> KPEPTDEEWELIKTVTEAHVATNAQGSHWKQKRKFLPEDIGQAPIVNAPEGGKVDLEAFSHFTKIITPAITRVVDFAKKLPMFCELPCEDQIILLKGCCMEIMSLRAAVRYDPESET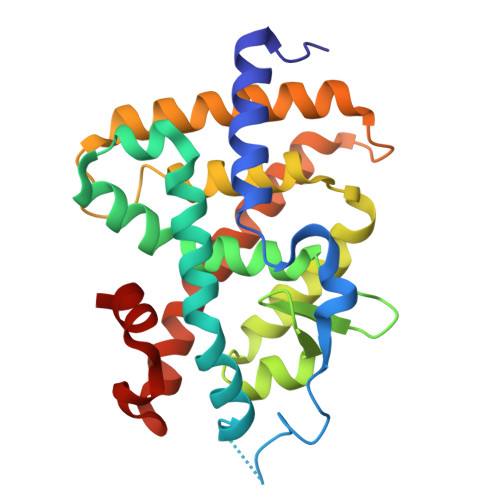LTLNGEMAVTRGQLKNGGLGVVSDAIFDLGMSLSSFNLDDTEVALLQAVLLMSSDRPGLACVERIEKYQDSFLLAFEHYINYRKHHVTHFWPKLLMKVTDLRMIGACHASRFLHMKVECPTELFPPLFLEVFE3-[(4-methoxyphenyl)methylsulfanyl]-5-(2-methylpropyl)-4-(phenylmethyl)-1,2,4-triazole 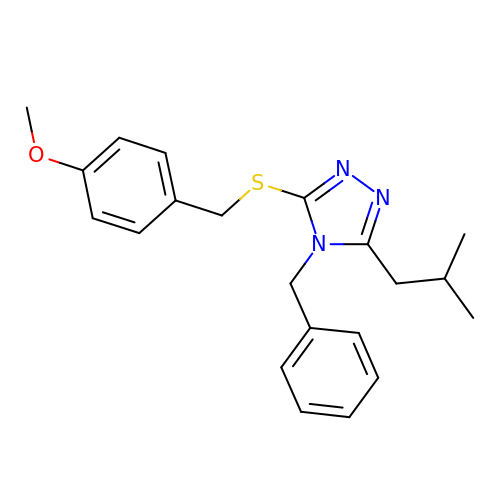| C21 H25 N3 O S | WYMPXNJKMFASMX-UHFFFAOYSA-N>GSHVANSVLFPCKYASSGCEITLPHTEKADHEELCEFRPYSCPCPGASCKWQGSLDAVMPHLMHQHKSITTLQGEDIVFLATDINLPGAVDWVMMQSCFGFHFMLVLEKQEKYDGHQQFFAIVQLIGTRKQAENFAYRLE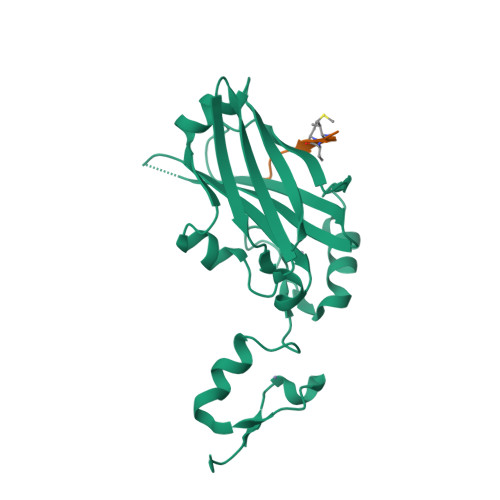LNGHRRRLTWEATPRSIHEGIATAIMNSDCLVFDTSIAQLFAENGNLGINVTISMC[2x];>XKLRPVAMVRPTVR[2x]> IVGGYTCGANTVPYQVSLNSGYHFCGGSLINSQWVVSAAHC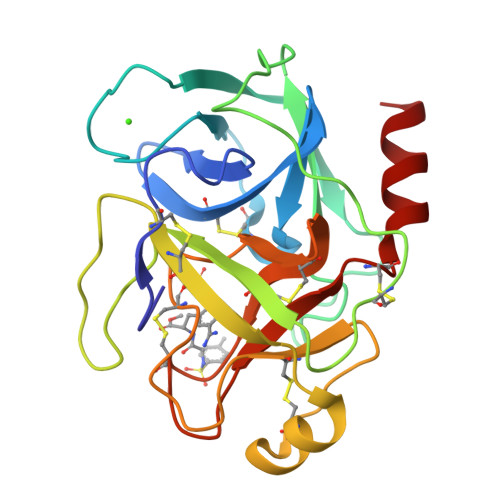YKSGIQVRLGEDNINVVEGNEQFISASKSIVHPSYNSNTLNNDIMLIKLKSAASLNSRVASISLPTSCASAGTQCLISGWGNTKSSGTSYPDVLKCLKAPILSDSSCKSASSWIITSNMFCAGYLEGGKDSCQGDSGGPVVCSGKLQGIVSWGSGCAQKNKPGVYTKVCNYVSWIKQTIASN> MVHYYRLSLKSRQKAPKIVNSKYNSILNIALKNFRLCKKHKTKKPVQILALLQEIIPKSYFGTTTNLKRFYKVVEKILTQSSFECIHLSVLHKCYDYDAIPWLQNVEPNLRPKLLLKHNLFLLDNIVKPIIAFYYKPIKTLNGHEIKFIRKEEYISFESKVFHKLKKMKYLVEVQDEVKPRGVLNIIPKQDNFRAIVSIFPDSARKPFFKLLTSKIYKVLEEKYKTSGSLYTCWSEFTQKTQGQIYGIKVDIRDAYGNVKIPVLCKLIQSIPTHLLDSEKKNFIVDHISNQFVAFRRKIYKWNHGLLQGDPLSGCLCELYMAFMDRLYFSNLDKDAFIHRTVDDYFFCSPHPHKVYDFELLIKGVYQVNPTKTRTNLPTHRHPQDEIPYCGKIFNLTTRQVRTLYKLPPNYEIRHKFKLWNFNNQISDDNPARFLQKAMDFPFICNSFTKFEFNTVFNDQRTVFANFYDAMICVAYKFDAAMMALRTSFLVNDFGFIWLVLSSTVRAYASRAFKKIVTYKGGKYRKVTFQCLKSIAWRAFLAVLKRRTEIYKGLIDRIKSREKLTMKFHDGEVDASYFCKLPEKFRFVKINRKASI

Telomerase is a multicomponent, ribonucleoprotein enzyme that includes a catalytic telomerase reverse transcriptase (TERT) protein and a noncoding RNA molecule that serves as the template for synthesis of telomere DNA. Telomerase functions as a unique RT that uses a specialized, noncoding RNA as a template for telomere DNA synthesis. In highly proliferative tissues (e.g., during embryogenesis, germline and stem cells), telomerase, the enzyme that synthesizes telomere ends, is reactivated to extend telomere DNA to counterbalance telomere attrition. Although TERT contains additional domains, its catalytic core is structurally homologous to the RT domain of HIV-1.

In doing so, we have identified 5-methylcarboxyl-indolyl-2′-deoxyriboside 5′-triphosphate (5-MeCITP) as an inhibitor of telomerase activity. To identify the precise interactions that govern 5-MeCITP binding to telomerase, we crystalized the T. castaneum TERT-MeCITP complex along with a nucleotide hairpin that functionally mimics the telomerase RNA template-telomere DNA substrate. The structure of the complex refined to 2.8 Å identifies density corresponding to an unpolymerized 5-MeCITP residing in the active site of the enzyme. The triphosphate group of 5-MeCITP is coordinated by two metal ions in a manner that is structurally similar to that of a nonhydrolyzable nucleotide analog bound to the active site of other polymerases. The modified nucleobase of 5-MeCITP adopts a noncanonical configuration in which it is rotated 180° as compared with the expected orientation of a native dNTP forming Watson-Crick base pairs with the RNA template. This configuration is very likely governed by an inability to properly base pair with RNA combined with selective interactions formed between the methylcarboxyl moiety of 5-MeCITP and TERT. Specifically, the methylcarboxyl moiety occupies a hydrophobic patch formed between motifs 1, 2 of the fingers domain and T-motif in the TRBD. The positioning of the methylcarboxyl group of 5-MeCITP is coordinated by interactions with Ile187 and Ile196 of motifs 1 and 2 and with Leu141 of the T-motif of T. castaneum TERT. The unique positioning of the modified nucleotide coincides with a displacement of the nucleobase of the template away from its canonical position. The α-phosphate of 5-MeCITP is situated at a distance that is approximately 5 Å from the nucleophilic 3′-hydroxyl group of the terminal dATP of the ssDNA that is being extended and is therefore too far for nucleophilic attack and incorporation into the 3′ end of the DNA.>MTLTTVIDIGNFSTKYAYKDKKQIKVGSFPSILHSYKPLEDYEGMERVEYNGLDYYVGETVKNFYFGREEQMYFGNTRKGHMEGQIRLVYALYTIFKETGKKEFNLILTCPYESMVTDKKYFVQHFEGEREVIVEGKSFKFTVHNIVMAAEGLGALNFSDSLNCVIVDAGSKTLNVLYLINGSISKMDSHTINGGTIDNSIMDL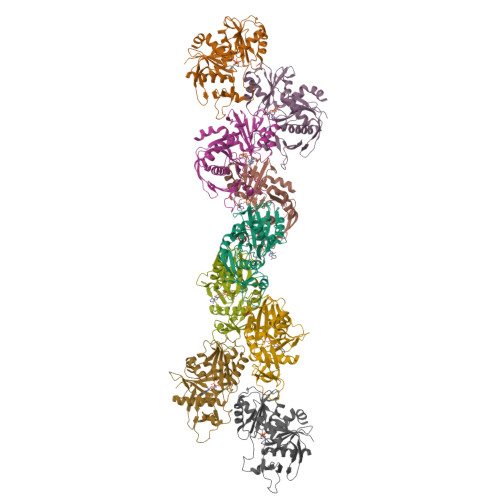AKTFAKTCSNIDYDYPIVCTGGKAEEMKECLENVGYSTVSSAELGEDKPSYYVNSVGLLLKYGRKFEEMFA[9x]>MTMASVPASRYLTDMTLEEMSRDWSMLIPKQKVAGPLCIRMDQAIMDKNIILKANFSVIFDRLETLILLRAFTEEGAIVGEISPLPSLPGHTAEDVKNAVGVLIGGLEWNDNTVRVSETLQRFAWRSSNENGRPPLTPKQ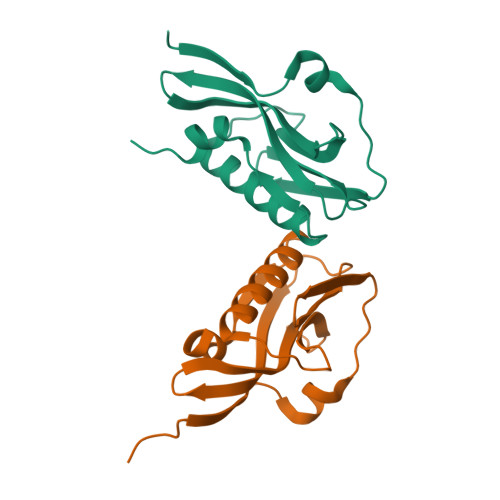KREMAGTIRSEV[2x]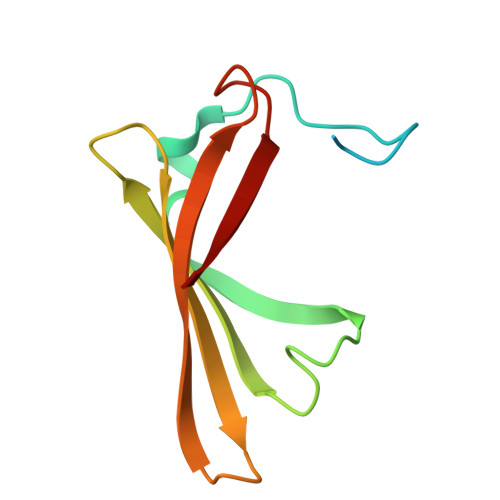> MGHHHHHHLESTSLYKKSSSTPPRGVTVVNNFDAKRYLGTWYEIARFDHRFERGLEKVTATYSLRDDGGLNVINKGYNPDRGMWQQSEGKAYFTGAPTRAALKVSFF>[2x]GGPYLQILEQPKQRGFRFRYVCEGPSHGGLPGASSEKNKKSYPQVKICNYVGPAKVIVQLVTNGKNIHLHAHSLVGKHCEDGVCTVTAGPKDMVVGFANLGILHVTKKKVFETLEARMTEACIRGYNPGLLVHSDLAYLQAEGGGDRQLTDREKEIIRQAAVQQTKEMD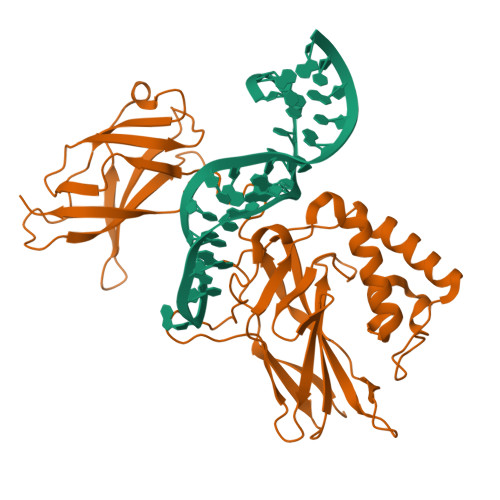LSVVRLMFTAFLPDSTGSFTRRLEPVVSDAIYDSKAPNASNLKIVRMDRTAGCVTGGEEIYLLCDKVQKDDIQIRFYEEEENGGVWEGFGDFSPTDVHRQFAIVFKTPKYKDVNITKPASVFVQLRRKSDLETSEPKPFLYYPEIKDKEEVQRKRQK>[4x]MIKQRTLKNIIRATGVGLHSGEKVYLTLKPAPVDTGIVFSRTDLDPVVEIPARAENVGETTMSTTLVKGDVKVDTVEHLLSAMAGLGIDNAYVELSASEVPIMDGSAGPFVFLIQSAGLQEQEAAKKFIRIKREVSVEEGDKRAVFVPFDGFKVSFEIDFDHPVFRGRTQQASVDFSSTSFVKEVSRARTFGFMRDIEYLRSQNLALGGSVENAIVVDENRVL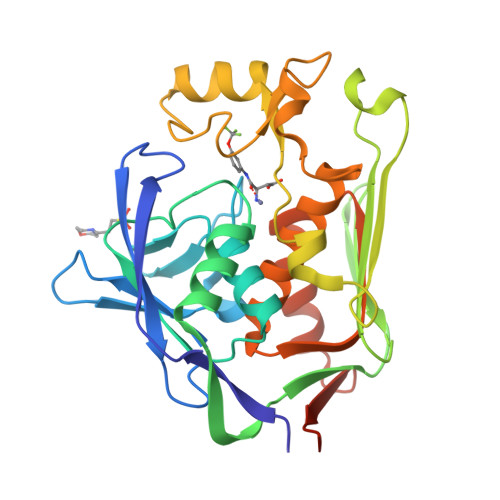NEDGLRYEDEFVKHKILDAIGDLYLLGNSLIGEFRGFKSGHALNNQLLRTLIADKDAWEVVTFEDARTAPISYMRP>GPGQKKRLSVSAEAYGDWNKKIDNFIPKVYKKDEKEKAKIREALNESFLFNHLNKKEFEIIVNAFFDKNVEKGVNIINEGDYGDLLYVIDQGEVEIYKTKENNKKEVLTVLKSKDVFGELALLYNSKRAATATALTKCHLWALDRESFTYIIKDMVAKKRKMYEDILSHVNILKDMDPYERCKVADCLKSKSYNDGEIIIKEGEEGDTFFILIDGNAVASKDNKVIKTYTKGDYFGELALLKNKPRAATIKAQNFCQVVYLDRKSFKRLLGPIEDILHRNVEN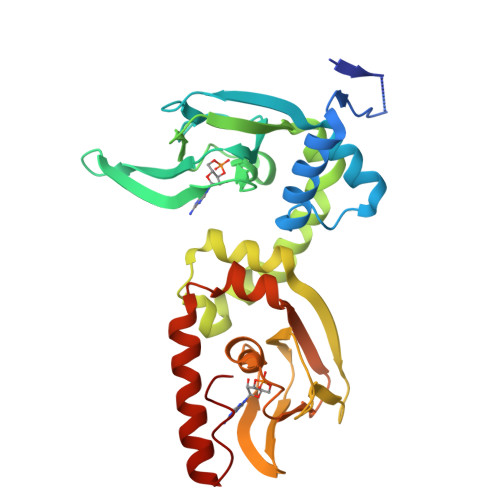YKKVLNELGLDTTCIDEN[2x]>[15x]MELFDENYYAKAVANIIGEVKDPIMYKWFSPDQIEDVDLQMGYQKTVKWDAFLNANPTTIANEVNTISTIGFSSEVVRLNYLKLQYKFRHLKQTSEKFYTSDSYIGDINNNLLPFAQAYKLASSEIIKLINHFVLTGTVSIQKDGKNQKRLLPNMYGLLNMPEQIKEEVASGDKDKMDKIFEKIEAGLSKLELGDEFSTPMMVIVDPATSLKLVKPYAAAQGAASSCEKWEDVLIQTIKAINNREDVYIETSNLLKHKILIYPLNSELIKFKPSKYMLPTPNEQVDKDSTD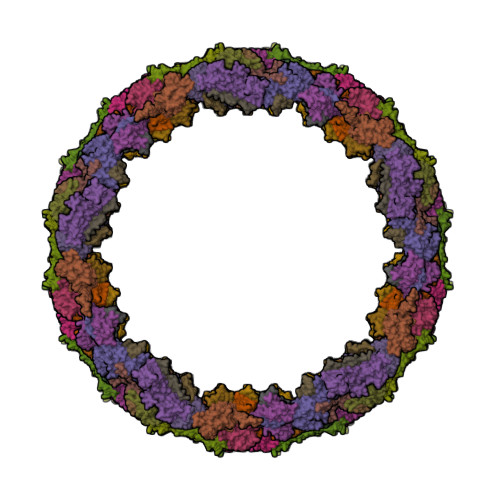VAHSYIDFVLGGLLATRKTILQVNIKQS;>MSDITKIKQEFDKKVAEIQALMKNPQQDSGLLSNSIDFRDQNLIFSNSGGVCTSSKDKIENYPAKGYPYKRGVKLSFGDGTTELEVEAGGGDDLYGVCSDIDEFSGMATVIPITNNFTGYLTLKKDGQNGVNPGDKLNFNQHGELEKVTGAQKSVNAIALSKAHKLTEDLFIVLASVFGNRAIKG[8x];>[4x]MGDTTQLVKEYQEKRSKLEKFMKNPQHDASLLSNSNEFRDKNVEFFASGGTRTSKFDKLENHPFLGYPYKRGVKRVIQEAQDNQSHYEPHVEAGGGEDLYGICIDIDEFSKTATIVPITNNFEGYLVAKDSTVKVKDKLIFNKDGALEKVTGAPNKATINATALTDAKQISNEVYLVKVAVFGNKAMSRN;>MTEKEEKEDLQAQDKEEQQIKADTKVISVQEFEEYMRFKEQANSKSKETSRDLSINERITKELAEVEERERIEKQLLLEAERINEIDTLAKAHLSNHFNKEVLLAKGYTLKDIMQAQRRELVRKFVPIEQIKAIAKVSDISHIDGEILEQLVSLAKVNIKLRKNASSSSSSVDSIKGNIAIKSEERASLLDSNFVPINFTEFVQAISNTYKQRRIQFYENLKRHKRTSIA[15x]> GSHMVPAALPQLTPTLVSLLEVIEPEVLYAGYDSSVPDSAWRIMTTLNMLGGRQVIAAVKWAKAIPGFRNLHLDDQMTLLQYSWMSLMAFALGW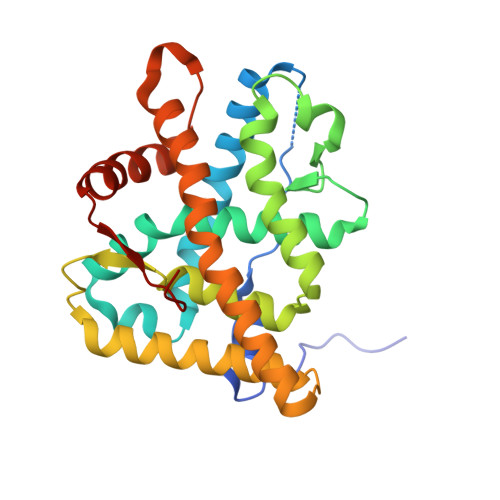RSYRQASGNLLCFAPDLIINEQRMTLPCMYDQCKHMLFISTELQRLQVSYEEYLCMKTLLLLSSVPKEGLKSQELFDEIRMTYIKELGKAIVKREGNSSQNWQRFYQLTKLLDSMHDVVENLLSYCFQTFLDKSMSIEFPEMLAEIITNQIPKYSNGNIKKLLFHQK>[2x]MSTQYETQGYTINNAGRRLVVDPITRIDGHMRCEVNINDQNVITNAVSCGTMFRGLEIILQGRDPRDAWAFVERICGVCTGVHALASVYAIEDAIGIKVPDNANIIRNIMLATLWCHDHLVHFYQLAGMDWIDVLDALKADPRKTSELAQSLSSWPKSSPGYFFDVQNRLKKFVEGGQLGIFRNGYWGHPQYKLPPEANLMGFAHYLEALDFQREIVKIHAVFGGKNPHPNWIVGGMPCAINIDESGAVGAVNMERLNLVQSIITRTADFINNVMIPDALAIGQFNKPWSEIGTGLSDKCVLSYGAFPDIANDFGEKSLLMPGGAVINGDFNNVLPVDLVDPQQVQEFVDHAWYRYPNDQVGRHPFDGITDPWYNPGDVKGSDTNIQQLNEQERYSWIKAPRWRGNAMEVGPLARTLIAYHKGDAATVESVDRMMSALNLPLSGIQSTL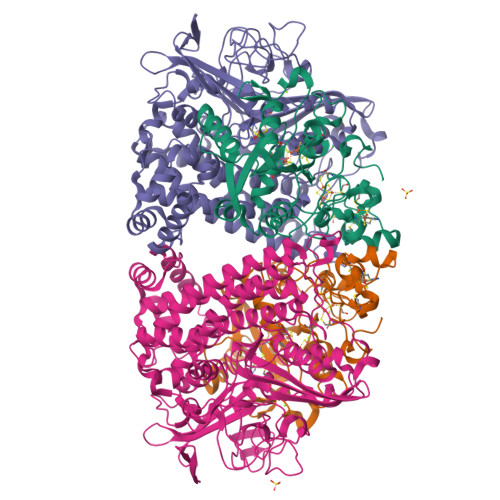GRILCRAHEAQWAAGKLQYFFDKLMTNLKNGNLATASTEKWEPATWPTECRGVGFTEAPRGALGHWAAIRDGKIDLYQCVVPTTWNASPRDPKGQIGAYEAALMNTKMAIPEQPLEILRTLHSFDPCLACSTH;>[2x]LENKPRIPVVWIHGLECTCCTESFIRSAHPLAKDVILSLISLDYDDTLMAAAGTQAEEVFEDIITQYNGKYILAVEGNPPLGEQGMFCISSGRPFIEKLKRAAAGASAIIAWGTCASWGCVQAARPNPTQATPIDKVITDKPIIKVPGCPPIPDVMSAIITYMVTFDRLPDVDRMGRPLMFYGQRIHDKCYRRAHFDAGEFVQSWDDDAARKGYCLYKMGCKGPTTYNACSSTRWNDGVSFPIQSGHGCLGCAENGFWDRGSFYSRVVDIPQMGTHSTADTVGLTALGVVAAAVGVHAVASAVDQRRRHNQQPTETEHQPGNEDKQARSHHHHHH>[2x]PFVNKQFNYKDPVNGVDIAYIK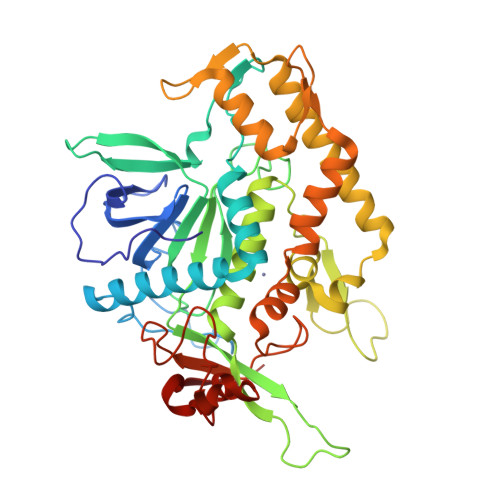IPNAGQMQPVKAFKIHNKIWVIPERDTFTNPEEGDLNPPPEAKQVPVSYYDSTYLSTDNEKDNYLKGVTKLFERIYSTDLGRMLLTSIVRGIPFWGGSTIDTELKVIDTNCINVIQPDGSYRSEELNLVIIGPSADIIQFECKSFGHEVLNLTRNGYGSTQYIRFSPDFTFGFEESLEVDTNPLLGAGKFATDPAVTLAHELIHAGHRLYGIAINPNRVFKVNTNAYYEMSGLEVSFEELRTFGGHDAKFIDSLQENEFRLYYYNKFKDIASTLNKAKSIVGTTASLQYMKNVFKEKYLLSEDTSGKFSVDKLKFDKLYKMLTEIYTEDNFVKFFKVLNRKTYLNFDKAVFKINIVPKVNYTIYDGFNLRNTNLAANFNGQNTEINNMNFTKLKNFTPG Here, we investigated the biochemical, structural, and dynamic properties of the enzyme complex responsible for vitamin B6 (pyridoxal 5-phosphate, PLP) biosynthesis in S. aureus, which comprises enzymes SaPdx1 and SaPdx2. A multimeric assembly of two enzymes, Pdx1 and Pdx2, synthesizes pyridoxal 5-phosphate (PLP), the active form of vitamin B6, as well as its vitamers. Pdx2 has glutaminase activity, converting L-glutamine into L-glutamate and an ammonia molecule. The latter is delivered to Pdx1, which synthesizes PLP using ammonia, ribose 5-phosphate (R5P), and glyceraldehyde 3-phosphate (G3P).

However, Strohmeier and coworkers observed that a mutation in one amino acid from the catalytic site of BsPdx2, H170N (H165N in SaPdx2), stabilizes the Pdx1/Pdx2 complex in a fully saturated form, enabling structural analysis. The phaser found a solution with a final translation function Z-score/a log-likelihood gain of 18.5/1565, containing 12 SaPdx1 and 11 SaPdx2mut. However, during the refinement, an electron density for the 12th SaPdx2mut chain allowed the tracing of the chain, although with missing parts. The model was refined in Phenix.refine, and the final model was validated with MolProbity. The final model for the SaPLPmut complex showed remarkable structural conservation of the SaPdx1 dodecamer with minimal structural rearrangements after SaPdx2mut binding, as suggests the comparison of Figures 4D and 7A. According to PDBePISA, the 12 interfaces among SaPdx1 and SaPdx2mut have an average interface area of approx. 1424 Å2, with 23 hydrogen bonds and ten salt bridges, supporting the formation of the Pdx1–Pdx2 complex. A glutamine residue was observed in the active site of SaPdx2mut. The Nε atom from glutamine interacts with the catalytic cysteine C75 (2.3 Å), as shown in Figure 7B. Unexpectedly, for one of the 12 SaPdx2mut molecules bound to SaPdx1, the electron density was observed to be rather weak.

>[12x]GAMSKIIGSDRVKRGMAEMQKGGVIMDVVNAEQARIAEEAGAVAVMALERVPSDIRAAGGVARMANPKIVEEVMNAVSIPVMAKARIGHITEARVLEAMGVDYIDESEVLTPADEEYHLRKDQFTVPFVCGCRNLGEAARRIGEGAAMLRTKGEPGTGNIVEAVRHMRQVNSEVSRLTVMNDDEIMTFAKDIGAPYEILKQIKDNGRLPVVNFAAGGVATPQDAALMMELGADGVFVGSGIFKSEDPEKFAKAIVQATTHYQDYELIGRLASELGTAMKGLDINQLSLEERMQERGW;>GAMKIGVLALQGAVREHIRHIELSGHEGIAVKKVEQLEEIEGLILPGGESTTLRRLMNLYGFKEALQNSTLPMFGTCAGLIVLAQDIVGEEGYLNKLNITVQRNSFGRQVDSFETELDIKGIATDIEGVFIRAPHIEKVGQGVDILCKVNEKIVAVQQGKYLGVSFNPELTDDYRVTDYFINHIVKKA[12x]>[2x]GPHMASLVIISTLDGRIAALDPENHGKKQWDLDVGSGSLVSSSLSKPEVFGNKMIIPSLDGALFQWDRDRESMETVPFTVESLLESSYKFGDDVVLVGGKSLTTYGLSAYSGKVRYICSALGCRQWDSDEMEQEEDILLLQRTQKTVRAVGPRSGNEKWNFSVGHFELRYIPDMETRAGFIESTFKPNENTEESKIISDVEEQEAAIMDIVIKVSVADWKVMAFSKKGGHLEWEYQFCTPIASAWLLKDGKVIPISLFDDTSYTSNDDVLEDEEDIVEAARGATENSVYLGMYRGQLYLQSSVRI

The unfolded protein response is an important cell signaling system that detects the accumulation of misfolded proteins within the endoplasmic reticulum (ER) and carries out a cellular response that attempts to rectify the imbalance. There are three sensor/transducer proteins: Ire1, PERK, and Atf6, that are critical for initiating mammalian UPR cell signaling and give rise to three separate branches of the response. All three proteins have a luminal sensor/transducer domain that in concert with BiP is vital for sensing ER stress, an ER transmembrane region, and a cytosolic domain that propagates the UPR signal (Bertolotti et al, 2000; Schröder & Kaufman, 2005; Ron & Walter, 2007; Zhang & Kaufman, 2008). In an attempt to shed new light upon the mechanism of UPR activation and to rationalize the differences between Ire1 luminal domain structures, we determined the crystal structures of PERK luminal domains in two different states: one state is the previously characterized dimer arrangement as seen with Ire1, and the other state is a novel tetramer arrangement.

An optimized human PERK luminal domain construct encompassing residues 105–403 was expressed and purified with cleavable N-terminal His-tag in E. coli. To overcome this, we used a tungsten-derivatized multi-anomalous dispersion (MAD) dataset which yielded a good quality electron density map, from which we were able to build the structure of human PERK luminal domain, and subsequently used this as a molecular replacement model for the mouse PERK luminal domain. The human PERK luminal domain structure forms a ring-type tetramer architecture. The individual monomers are arranged along a twofold rotation axis forming two sets of dimers A–B and C–D. Each dimer presents an inward-facing concave surface that intimately locks together at both ends to create a space in the center of the ring tetramer (Fig1A and B). There are substantial contacts between monomers within the tetramer interface, with the key feature being a helix swapped between monomers; such secondary structure swap motifs are indicative of a transient interface (Ali et al, 2006; Czabotar et al, 2013; Tan et al, 2014). The salient feature of the tetramer interface is the α2 helix being swapped between opposing monomers that results in a total of 2,500 Å of solvent-accessible surface being buried, making this interface more substantial than the dimerization interface. The swapped α2 helix resides in a cleft created by β5–β7 and β18–β19 as part of the tetramer subdomain. The interface comprises predominantly hydrophobic interactions with a number of hydrogen bonds that also contribute to the interface between monomers. The electrostatic potential of α2 helix is positive while that of the cleft is negative. However, analysis of human PERK luminal domain protein by analytical ultra centrifugation (AUC) revealed a significant tetramer species that exists in equilibrium with dimer in solution, with a dimer to tetramer ratio of 3:2 (Fig5A).HadA is a flavin-dependent monooxygenase catalyzing hydroxylation plus dehalogenation/denitration, which is useful for biodetoxification and biodetection. HadA belongs to the class D two-component flavin-dependent monooxygenases, which use reduced FAD (FADH–) as a substrate. The initial and committing step of the had pathway catalyzed by HadA monooxygenase is hydroxylation with removal of either halide substituents (F, Cl, Br, or I) from HPs or a nitro group (-NO2) from NP. Each protomer is composed of three domains: the N-terminal domain (residues 1–146), the β-sheet domain (residues 147–275), and the C-terminal domain (residues 276–517).

We also solved the structure of the HadAPhe441Val−FADH–−4NP complex at 2.3-Å resolution. Although 4NP can still bind to this variant, the quadruple π-stacking motif was disrupted. The overall structure of the ternary complex of HadAPhe441Val is very similar to that of HadAWT (RMSD of 0.143) without any significant changes in the active site area. In contrast, the signals and amplitude of both A380 and A450 in both HadAPhe441Val and HadAPhe441Leu were independent of 4CP concentrations under the same conditions as HadAWT, indicating that the binding of 4CP does not prevent C4a-hydroperoxy-FAD formation. All data suggest that no substrate inhibition via dead-end complex formation was observed in these HadAPhe441 variants, which are void of the quadruple π-stacking complex at the subunit interface. Of interest, the complexes of HadAPhe441 variants and 4NP (in which 4NP can bind but the quadruple π-stacking is absent) showed increased Tm values (ΔTm) of only around 1.5 to 2.1 °C. Therefore, the Tm results imply that, upon 4NP binding at the subunit interface, especially with the quadruple π-stacking found in the HadAWT, the quaternary structures of HadA are likely more rigid than the apoenzyme forms. The difference between the structures of HadAWT and HadAPhe441Val around the subunit interface areas and Tm values clearly explain how the dead-end complex is stabilized in HadAWT but not HadAPhe441Val. The rates of 4NP conversion by HadAPhe441Val, HadAPhe441Leu, and HadAPhe441Ile were 21 ± 8%, 24 ± 13%, and 17 ± 10% greater than that of HadAWT, respectively (p-value < 0.05) (inset). The data indicate that alteration of Phe441, which removes the quadruple π-stacking interactions and, thus, dead-end complex formation ability, indeed improved biocatalysis by HadA.

>MIRTGTQYLESLNDGRNVWVGNEKIDNVATHPKTRDYAQRHADFYDLHHRPDLQDVMTYIDEGGQRRAMQWFGHRDKEQLRRKRKYHETVMREMAGASFPRTPDVNNYVLTTYIDDPAPWETQSIGDDGHIKAGKIVDFIRYAREHDLNCAPQFVDPQMDRSNPDAQERSPGLRVVEKNEKGIVVNGVKAIGTGVAFADWIHIGVFFRPGIPGDQVIFAATPVNTPGVTIVCRESLVKDDKVEHPLAAQGDELDGMTVFENVFIPWSHVFHIGNPNHAKLYPQRVFDWLHYHALIRQMVRAELVAGLAVLITEHIGTNKIPAVQTRVAKLIGFHQAMLAHLIASEELGFHTPGGHYKPNILIYDFGRALYLENFSQMIYELVDLSGRSALIFASEDQWNDDKLNGWFERMNNGPVGRPHDRVKIGRVIRDLFLTDWGSRLVVFENFNGTPLQGIRMLTMQRAEFSGSGPYGKLARQVCGIDSAVTDDTEYRKTADYAKALDAARHQEEVALAGAMAI[4x]>AYDRAITVFSPDGRLFQVEYAREAVKKGSTALGMKFANGVLLISDKKVRSRLIEQNSIEKIQLIDDYVAAVTSGLVADARVLVDFARISAQQEKVTYGSLVNIENLVKRVADQMQQYTQYGGVRPYGVSLIFAGIDQIGPRLFDCDPAGTINEYKATAIGSGKDAVVSFLEREYKENLPEKEAVTLGIKALKSSLEEGEELKAPEIASITVGNKYRIYDQEEVKKFL[7x];>[7x]TTTVGITLKDAVIMATERRVTMENFIMHKNGKKLFQIDTYTGMTIAGLVGDAQVLVRYMK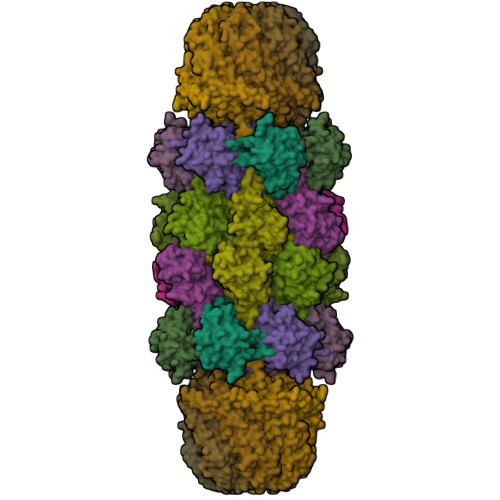AELELYRLQRRVNMPIEAVATLLSNMLNQVKYMPYMVQLLVGGIDTAPHVFSIDAAGGSVEDIYASTGSGSPFVYGVLESQYSEKMTVDEGVDLVIRAISAAKQRDSASGGMIDVAVITRKDGYVQLPTDQIESRIRKLGLIL;>[7x]KRAALIQNLRDSYTETSSFAVIEEWAAGTLQEIEGIAKAAAEAHGVIRNSTYGRAQAEKSPEQLLGVLQRYQDLCHNVYCQAETIRTVIAIRIPEHKEADNLGVAVQHAVLKIIDELEIKTLGSGEKSGSGGAPTPIGMYALREYLSARSTVEDKLLGSVDAESGKTKGGSQSPSLLLELRQIDADFMLKVELATTHLSTMVRAVINAYLLNWKKLIQPRTGTDHMYS>[8x]M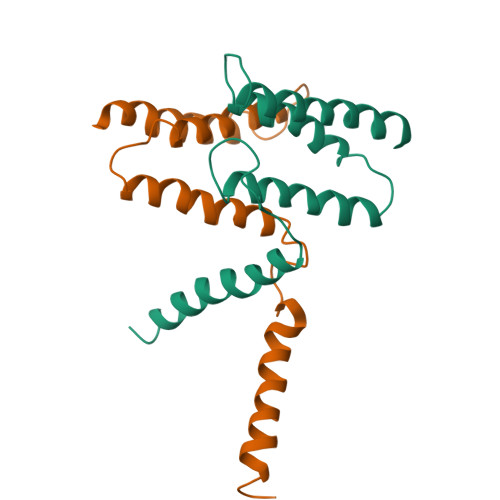NPYIYLGGAILAEVIGTTLMKFSEGFTRLWPSVGTIICYCASFWLLAQTLAYIPTGIAYAIWSGVGIVLISLLSWGFFGQRLDLPAIIGMMLICAGVLIINLLSRSTPH>[4x]LRSRRVDVMDVMNRLILAMDLMNRDDA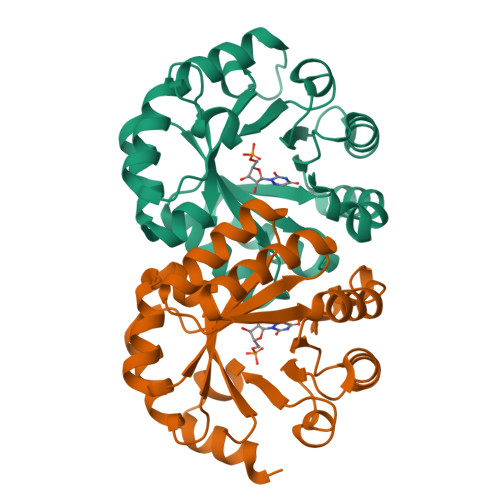LRVTGEVREYIDTVKIGYPLVLSEGMDIIAEFRKRFGCRIIADFKVADIPETNEKICRATFKAGADAIIVHGFPGADSVRACLNVAEEMGREVFLLTEMSHPGAEMFIQGAADEIARMGVDLGVKNYVGPSTRPERLSRLREIIGQDSFLISPGVGDPGETLRFADAIIVGASIYLADNPAAAAAGIIESIKDLLNP The glutaminase enzymes GAC and GLS2 catalyze the hydrolysis of glutamine to glutamate, satisfying the ‘glutamine addiction’ of cancer cells. All glutaminase enzymes share a catalytic domain containing identical active site residues and a conserved mechanism for hydrolyzing glutamine to glutamate. Here we demonstrate that the ability of GAC and GLS2 to form filaments is directly coupled to their catalytic activity and present their cryo-EM structures which provide a view of the conformational states essential for catalysis. Filament formation guides an ‘activation loop’ to assume a specific conformation that works together with a ‘lid’ to close over the active site and position glutamine for nucleophilic attack by an essential serine.

Therefore, we tested this prediction by taking advantage of our earlier finding that substituting an essential tyrosine residue within the enzyme active site of GAC does not disrupt substrate (glutamine) binding but prevents its hydrolysis to glutamate. We determined a 3.3 Å cryo-EM structure of the human GAC (Y466W) mutant which because it is defective for hydrolyzing glutamine to glutamate, assembled into a stable filament upon binding substrate and the anionic activator phosphate (Pi). Each successive tetramer is rotated ~51 degrees relative to the filament axis with the helical rise of ~68 Å. In both the GAC and GLS2 filament structures, each tetramer interacts with its immediate neighbor through an interface of six alpha helices on the lateral side of the catalytic domain near the lid loop that closes over the substrate binding site. In solving the cryo-EM structure for the GAC(Y466W) filament in the presence of glutamine and Pi, we were able to identify the Pi binding site within the dimer-dimer interface of each tetrameric unit where it interacts with Lys320 and thereby stabilizes the activation loop. However, in the filament structure of GAC, Pi interacts with Arg387, enabling it to form a salt bridge with Glu397 at the dimer-dimer interface, which together with the interactions of Pi with Tyr394 and Lys398, may be necessary for the glutaminase enzymes to undergo the dimer-to-tetramer transition, a prerequisite for filament formation and catalytic activity. Thus, the activation loops of each dimer within the filament fold in a compact manner, thereby bringing Phe318 of GAC (Tyr251 of GLS2) from each loop closer to the active site. When comparing the filament structures with those of the apo-enzyme, a second significant conformational change involves the lid loops, resulting in the insertion of Tyr249 of GAC (Tyr182 of GLS2) into the active site pockets. However, in the case of the GAC (Y466W) mutant, which binds Pi and substrate but cannot undergo catalysis, the filament persists and now the density of the lid loop within the terminal tetramer of the cryo-EM reconstruction remains intact.

>[12x]MMRLRGSGMLRDLLLRSPAGVSATLRRAQPLVTLCRRPRGGGRPAAGPAAAARLHPWWGGGGWPAEPLARGLSSSPSEILQELGKGSTHPQPGVSPPAAPAAPGPKDGPGETDAFGNSEGKELVASGENKIKQGLLPSLEDLLFYTIAEGQEKIPVHKFITALKSTGLRTSDPRLKECMDMLRLTLQTTSDGVMLDKDLFKKCVQSNIVLLTQAFRRKFVIPDFMSFTSHIDELYESAKKQSGGKVADYIPQLAKFSPDLWGVSVCTVDGQRHSTGDTKVPFCLQSCVKPLKYAIAVNDLGTEYVHRYVGKEPSGLRFNKLFLNEDDKPHNPMVNAGAIVVTSLIKQGVNNAEKFDYVMQFLNKMAGNEYVGFSNATFQSERESGDRNFAIGYYLKEKKCFPEGTDMVGILDFYFQLCSIEVTCESASVMAATLANGGFCPITGERVLSPEAVRNTLSLMHSCGMWDFSGQFAFHVGLPAKSGVAGGILLVVPNVMGMMCWSPPLDKMGNSVKGIHFCHDLVSLCNFHNYDNLRHFAKKLDPRREGGDQRHSFGPLDYESLQQELALKETVWKKVSPESNEDISTTVVYRMESLGEKS> PEGPEIRRAADNLEAAIKGKPLTDVWFAFPQLKTYQSQLIGQHVTHVETRGKALLTHFSNDLTLYSHNQLYGVWRVVDTGEEPQTTRVLRVKLQTADKTILLYSASDIEMLRPEQLTTHPFLQRVGPDVLDPNLTPEVVKERLLSPRFRNRQFAGLLLDQAFLAGLGNYLRVEILWQVGLTGNHKAKDLNAAQLDALAHALLEIPRFSYATRGQVDENKH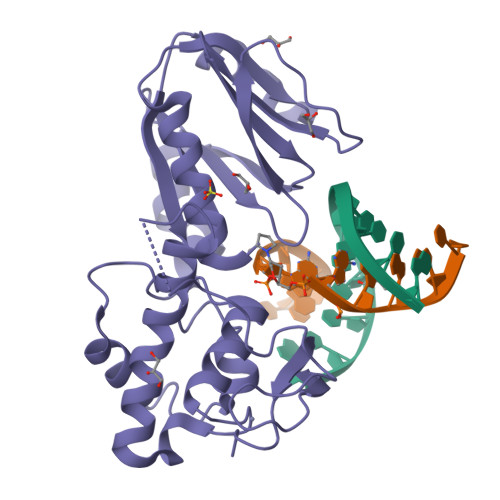HGALFRFKVFHRDGEPCERCGSIIEKTTLSSAPFYWCPGCQH>[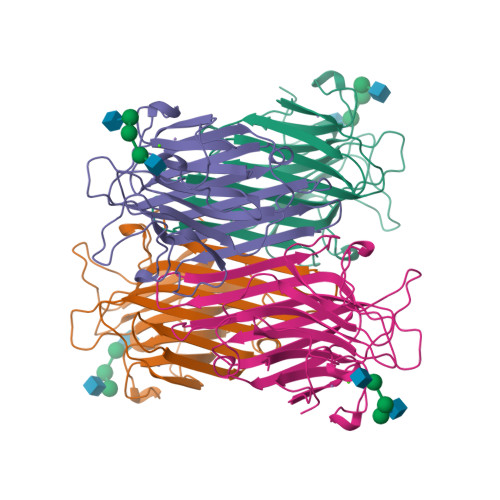8x]ADTIVAVELDTYPNTDIGDPSYPHIGIDIKSVRSKKTAKWNMQNGKVGTAHIIYNSVDKRLSAVVSYPNADSATVSYDVDLDNVLPEWVRVGLSASTGLYKETNTILSWSFTSKLKSNSTHETNALHFMFNQFSKDQKDLILQGDATTGTDGNLELTRVSSNGSPQGSSVGRALFYAPVHIWESSAVVASFEATFTFLIKSPDSHPADGIAFFISNIDSSIPSGSTGRLLGLFPDAN1-(3-{[(1R,4R,5S)-4-hydroxy-2-methyl-3-oxo-2-azabicyclo[3.1.0]hexan-4-yl]ethynyl}phenyl)-1H-pyrazolo[3,4-b]pyridine-3-carboxamide 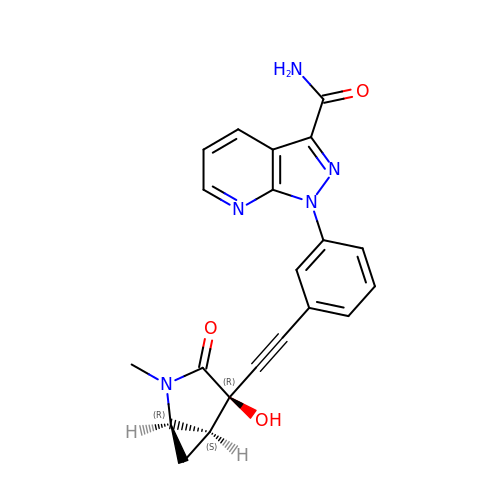| C21 H17 N5 O3 | GMAWUPHGBKLOEK-MRUHUIDDSA-N> LDKRQQVTLCEQYGYWSGNGYEINNNLWGRDSATSGWQCSYLDGSSDSGIQWHTTWEWQGGQHDVKSYVYSGKQFPRGQRITSINSMQTSVSWYYDTTNVRANVAYDIFTAADPNHVNSSGDYELMIWLAKYGDVQPI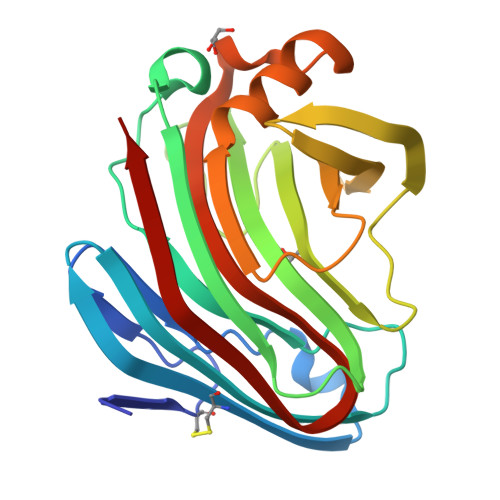GSPVGTVHVNGRNWELWIGMNGNMKVFSFIAPSPLNSWSGEVKEFFNYLQYNQGYPAGDQHLIVFQMGTEAFTGGPATMTVSHFSANIY>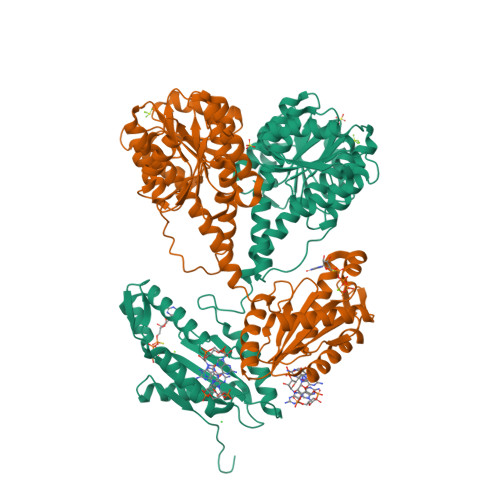[2x]SARILVVDDIEANVRLLEAKLTAEYYEVSTAMDGPTALAMAARDLPDIILLDVMMPGMDGFTVCRKLKDDPTTRHIPVVLITALDGRGDRIQGLESGASDFLTKPIDDVMLFARVRSLTRFKLVIDELRQREASGRRMGVIAGAAARLDGLGGRVLIVDDNERQAQRVAAELGVEHRPVIESDPEKAKISAGGPVDLVIVNAAAKNFDGLRFTAALRSEERTRQLPVLAMVDPDDRGRMVKALEIGVNDILSRPIDPQELSARVKTQIQRKRYTDYLRNNLDHSLELAVTDQLTGLHNRRYMTGQLDSLVKRATLGGDPVSALLIDIDFFKKINDTFGHDIGDEVLREFALRLASNVRAIDLPCRYGGEEFVVIMPDTALADALRIAERIRMHVSGSPFTVAHGREMLNVTISIGVSATAGEGDTPEALLKRADEGVYQAKASGRNAVVGKAAHHHHHH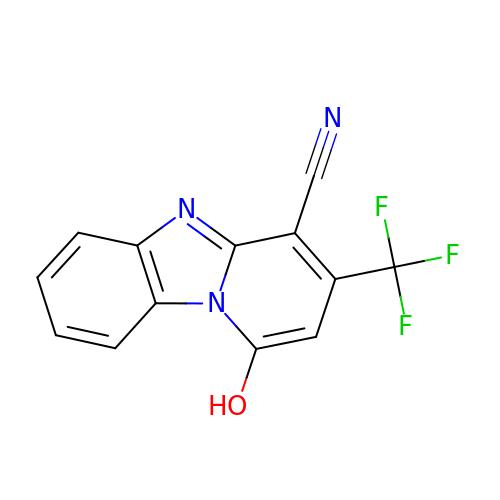1-Hydroxy-3-(trifluoromethyl)pyrido[1,2-a]benzimidazole-4-carbonitrile | C13 H6 F3 N3 O | NSMPADIWUYJQKF-UHFFFAOYSA-N>MASSVNELENWSKWMQPIPDNIPLARISIPGTHDSGTFKLQNPIKQVWGMTQEYDFRYQMDHGAR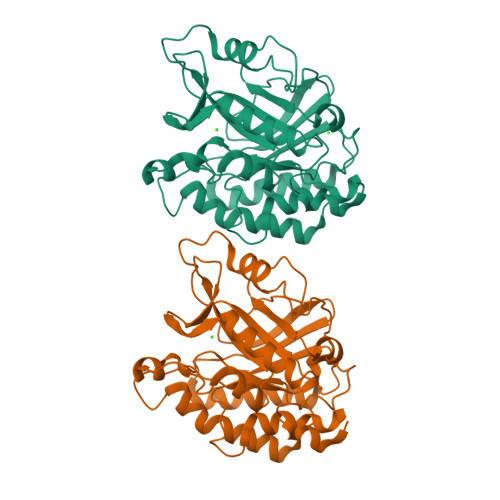IFDIDGRLTDDNTIVLHHGPLYLYVTLHEFINEAKQFLKDNPSETIIMSLKKEYEDMKGAEGSFSSTFEKNYFVDPIFLKTEGNIKLGDARGKIVLLKRYSGSNESGGYNNFYWPDNETFTTTVNQNVNVTVQDKYKVNYDEKVKSIKDTMDETMNNSEDLNHLYINFTSLSSGGTAWNSPYYYASYINPEIANDIKQKNPTRVGWVIQDYINEKWSPLLYQEVIRANKSLIKE[2x]>[2x]MEETPR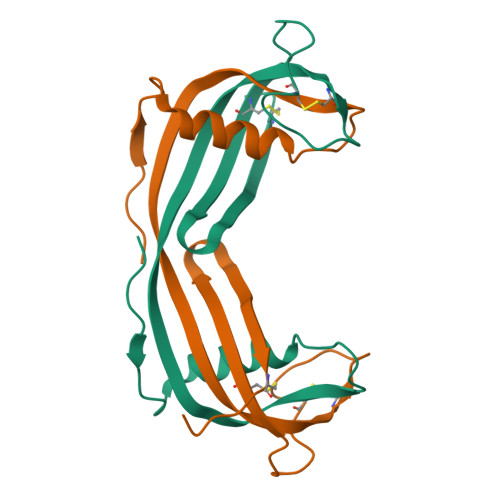LVGGWQKKPVDGNQLFTELAHFAVGNQVGDREFFDTVLEVIDAETQVVAGTNYRLTFKIAESTCRVTETYTKELCLPKTQDVKDTCTAVIYDVPWLNQRSVSSFTCGVNAAST> MELALRGGYRERSNQDDPEYLELAHYATSTWSAQQPGKTHFDTVVEVLKVETQTVAGTNYRLTLKVAESTCELTSTYNKDTCQANANAAQRTCTTVIYRN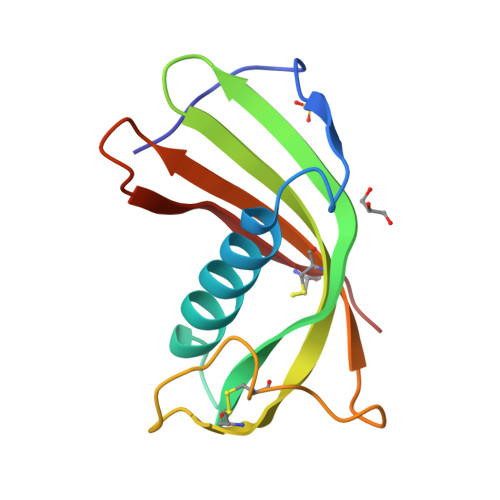LQGEKSISSFECAAA L-gamma-glutamyl-S-hexyl-L-cysteinylglycine | C16 H29 N3 O6 S | 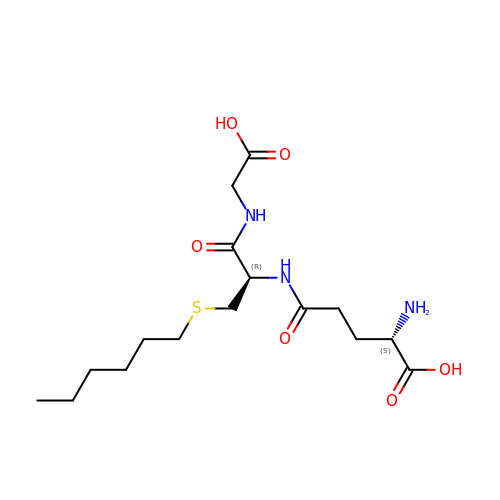HXJDWCWJDCOHDG-RYUDHWBXSA-N> GAMSTTSTTIQVIGAGLPRTGTNSMKKALEIIYSKPCYHMYEIIFKKQSDISIWQQLIDETHKTTSDKRKIYNGLNELLNGYIATTDLPSCSFYKELMTMYPNAKVLLTIRD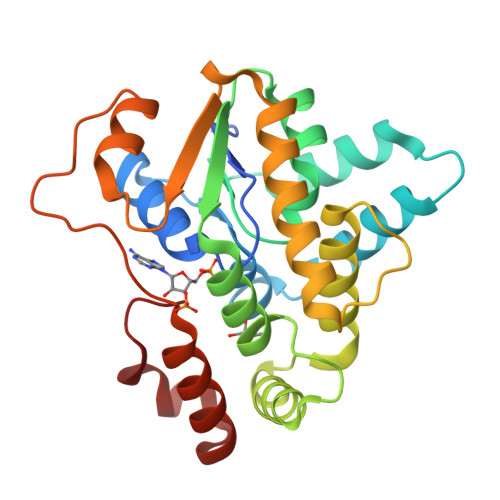KYDWLYSLRKVVLPKSTDPWKLKIEEGDQVLGIDSNFYKMSEDSLKFAFQKNHINLDDDEILLECYDEYNRLVQEIVPPERLLIHHLGDGWESLCQFLNVDIPNGISYPCANSHHQMTQLTEQLIKHKSLDDIIHMFPGLI> SPSAEECGYSDRVRSITLGNSTITTQECANVVVGYGVWPTYLKDEEATAEDQPTQPDVATCRFYTLESVMWQQS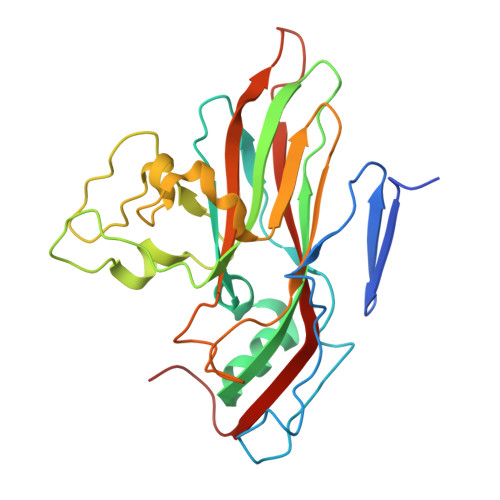SPGWWWKFPDALSNMGLFGQNMQYHYLGRAGYTIHVQCNASKFHQGCLLVVCVPEAEMGCATLANKPDPKSLSKGEIANMFESQNSTGETAVQANVINAGMGVGVGNLTIFPHQWINLRTNNSATIVMPYINSVPMDNMFRHNNFTLMVIPFAPLSYSTGATTYVPITVTVAPMCAEYNGLRLAGKQ>[3x]MGHHHHHHMSDKFSHITKDIT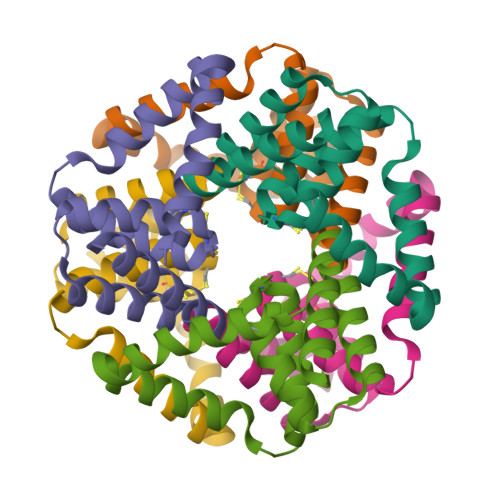TQLAKFRKEMPELMTGFSSLAQAATKDGALDKKTKELIAMALAVAKQCPGCIGFHSQTLVKLQATREELLETLGMAVYMGGGPSLMYAAEALEAFEEFSK>MVSFKRYELPPLPYNYNALEPYIIEEIMKLHHQKHHNTYVKGANAALEKIEKHLKGEIQIDVRAVMRDFSFNYAGHIMHTIFWPNMAPPGKGGGTPGGRVADLIEKQFGGFEKFKALFSAAAKTVEGVGWGVLAFDPLTEELRILQ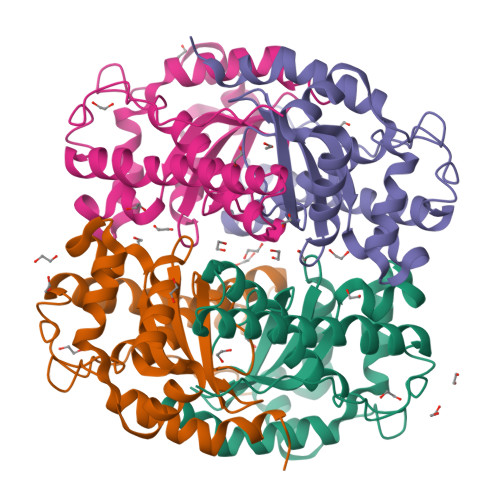VEKHNVLMTAGLVPILVIDVWEHAYYLQYKNDRGSYVENWWNVVNWDDVEKRLEQALNNAKPLYLLPQ[4x]6-DEOXYDAUNOMYCIN | C27 H29 N O9 | 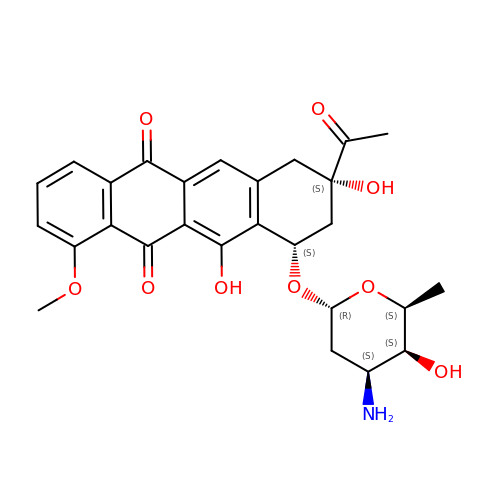ZCLQMQOBRBUQOR-GRRPPOEGSA-N> GSHMYANP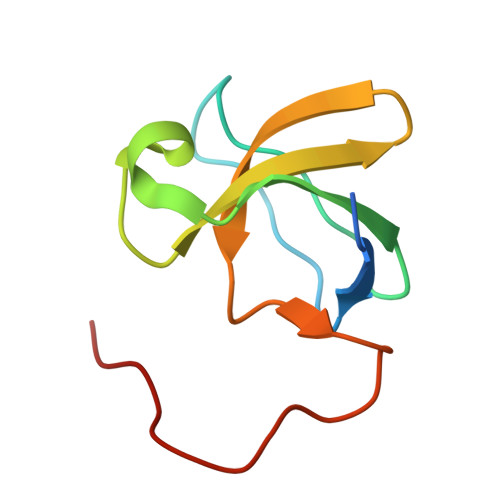VWTALFDYEPSGQDELALRKGDRVEVLSRDAAISGDEGWWAGQVGGQVGIFPSNYVSRGGGPPPPGPAVAEE>[2x]GIDPFTKTSLYESTLKNQTDLLKVTQSTVEDFRSTNQSFTRALEKDIANLPYQSLITEENIINNVGPILKYYRHSINALNVYLGLNNGKVLLSQKSNDAKMPELRDDLDIKTKDWYQEALKTNDIFVTPAYLDTVLKQYVITYSKAIYKDGKIIGVLGVDIPSEDLQNLVAKTPGNTFLFDQKNKIFAATNKELLNPSIDHSPVLNAYKLNGDNNFFSYKLNNEERLGACTKVFAYTACITESADIINKPIYKA

Small molecules in the environment can be sensed as attractants or repellents by a repertoire of chemoreceptors termed methyl-accepting chemotaxis proteins (MCPs) or transducer-like proteins (Tlps). Analysis of the crystal structure of the LBDs of C. jejuni Tlp1 and Tlp3 revealed that they have a double Cache (dCache; calcium channels and chemotaxis receptors) fold. dCache domains consist of two tandem subdomains (termed membrane-distal and membrane-proximal) that likely emerged through tandem segmental DNA duplication. We also discovered eight new small-molecule ligands that, in addition to isoleucine, signal through Tlp3 as attractants by binding directly to its LBD, and determined the crystal structures of the respective complexes. The hydrophobic side-chain binding pocket and the conserved protein residues that interact with the ammonium and carboxylate groups of the ligands determine the specificity of this chemoreceptor, which appears to have evolved as a receptor for natural non-polar amino acids.

To identify candidate signal molecules of this class, we generated a virtual library comprising ~2600 L-isoleucine analogues and screened it by docking into the known L-isoleucine binding site of Tlp3 LBD. The three water-soluble compounds with the lowest predicted free energy of binding (4-methyl-L-isoleucine, β-methyl-L-norleucine, and 3-methyl-L-isoleucine) were selected for the subsequent experiments. In the thermal shift assay, the ΔTm values for all three compounds (2.8 °C, 3.7 °C, and 2.0 °C) exceeded the 1.0 °C threshold, suggesting their direct binding to Tlp3 LBD. Among the non-natural amino acids, α-amino-N-valeric acid showed a slightly lower affinity for Tlp3 LBD (168 μM) than isoleucine and leucine, followed by β-methyl-L-norleucine (Kd = 294 μM), 4-methyl-L-isoleucine (Kd = 324 μM), and 3-methyl-L-isoleucine (Kd = 484 μM). The side chain of β-methyl-L-norleucine makes van der Waals contacts with the side chains of Tyr118, Leu128, Leu144, Trp151, and Val171 and approaches within 4.0 Å of the side chains of Gln130 and Asn116. Increasing the length of the carbon chain beyond five atoms decreases the binding affinity, as seen with β-methylnorleucine (Kd of 294 µM). Our crystallographic analysis provided a structural rationale for this phenomenon: the strongly hydrophobic side-chain-binding pocket can expand to accommodate molecules with the carbon backbone of up to five atoms in length, while longer linear side chains (such as that of β-methylnorleucine) are flipped to the outside of the pocket, which reduces favourable van der Waals contacts with the protein and, hence, lowers the binding affinity.> MARHGPPWSRLDAQQERDVRELVRGVAGLQDEADPNFQLALNFAWSNFRFHRFLDVNSHKIEKTIEGIYEKFVIHSDLSKAASWKRLTEEFLNAPLPSIKEIKTDAHYSILSLLLCLSDSPSNSSYVETPRNKEVEKKDDFDWGKYLMEDEEMDIGPYMDTPNWSEESEEENDQQPLSREDSGIQVDRTPLEEQDQNRKLDPCISWKDEPDDRSWLEHHVVHQYWTARPSQFPHSLHLHSNLAAVWDQHLYSSDPLYVPDDRVLVTETQVIRETLWLLSGVKKLFIFQLIDGKVTVRNNIIVTHLTHSCLRSVLEQIAAYGQVVFRLQEFIDEVMGHSSESMLPGSGSVPKKSTEAPFRTYQAFMWALYKYFISFKEELAEIEKCIINNDTTITLAIVVDKLAPRLSQLKVLHKVFSTGVAEVPPDTRNVVRASHLLNTLYKAILEYDNVGEASEQTVSLLFSLWVETV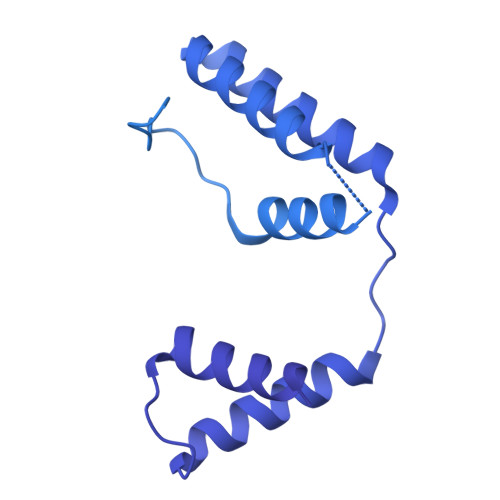RPYLQTVDEWIVHGHLWDGAREFIIQRNKNVPVNHRDFWYATYTLYSVSEKTENEEKMSDNASASSGSDQGPSSRQHTMVSFLKPVLKQIIMAGKSMQLLKNLQCAESTTCQAGARDAERKSLYTLFLESVQSRLRHGEDSTPQVLTEQQATKENLMKMQSIAESHLELDDVHDPLLAINFARMYLEQSDFHEKFAGGDVCVDRSSESVTCQTFELTLRSCLYPHIDKQYLDCCGNLMQTLKKDYRLVEYLQAMRNFFLMEGGDTMYDFYTSIFDKIREKETWQNVSFLNVQLQEAVGQRYPEDSSRLSISFENVDTAKKKLPVHILDGLTLSYKVPWPVDIVISLECQKIYNQVFLLLLQIKWAKYSLDVLLFGELVSTAEKPRLKEGLIHEQDTVAQFGPQKEPVRQQIHRMFLLRVKLMHFVNSLHNYIMTRILHSTGLEFQHQVEEAKDLDQLIKIHYRYLSTIHDRCLLREKVSFVKEAIMKVLNLALMFADGWQAGLGTWRMESIEKMESDFKNCHMFLVTILNKAVCRGSFPHLESLALSLMAGMEQS>[6x]GSHMPSRRMLHTMIRVGDLDRSI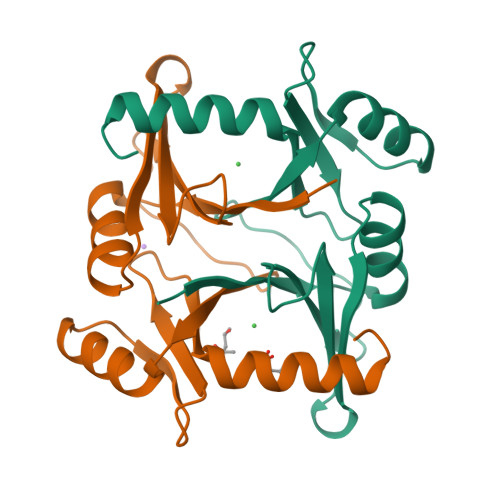KFYTERLGMKVLRKWDVPEDKYTLVFLGYGPEMSSTVLELTYNYGVTSYKHDEAYGHIAIGVEDVKELVADMRKHDVPIDYEDESGFMAFVVDPDGYYIELLNEKTMMEKAEADMKEQGTA> SMVKKTVRFGEQAAVPAIGLGTWYMGEHAAQRQQEVAALRAGIDHGLTVIDTAEMYADGGAEEVVGQAIRGLRDRVVLVSK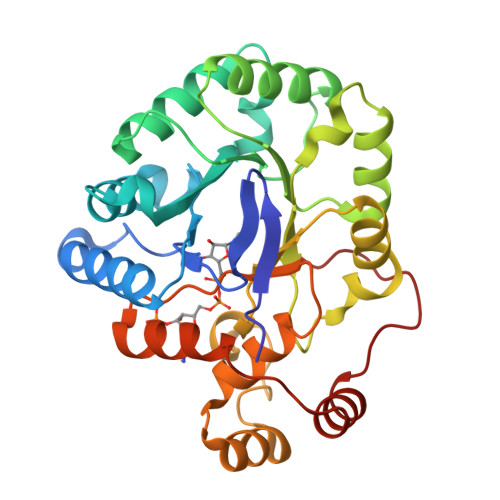VYPWHAGKAAMHRACENSLRRLQTDYLDMYLLHWRGDIPLQETVEAMEKLVAEGKIRRWGVSNLDTEDMQALWRTADGEHCATNQVLYHLASRGIEYDLLPWCQQHSLPVMAYCPLAQAGRLRDGLFQHSDIINMANARGITVAQLLLAWVIRHPGVLAIPKAASIEHVVQNAAALDIVLSGEELAQLDRLYPPPQRKTRLDMV(2R)-8-BENZYL-2-HYDROPEROXY-6-(4-HYDROXYPHENYL)-2-(4-IODOBENZYL)-7,8-DIHYDROIMIDAZO[1,2-A]PYRAZIN-3(2H)-ONE 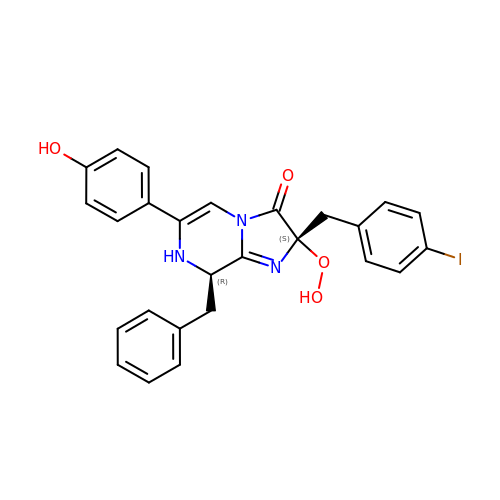| C26 H22 I N3 O4 | VKJBKKSOPAEBAT-GJZUVCINSA-N>[6x]MAASTGYVRLWGAARCWVLRRPMLAAAGGRVPTAAGAWLLRGQRTCDASPPWALWGRGPAIGGQWRGFWEASSRGGGAFSGGEDASEGGAEEGAGGAGGSAGAGEGPVITALTPMTIPDVFPHLPLIAITRNPVFPRFIKIIEVKNKKLVELLRRKVRLAQPYVGVFLKRDDSNESDVVESLDEIYHTGTFAQIHEMQDLGDKLRMIVMGHRRVHISRQLEVEPEEPEAENKHKPRRKSKRGKKEAEDELSARHPAELAMEPTPELPAEVLMVEVENVVHEDFQVTEEVKALTAEIVKTIRDIIALNPLYRESVLQMMQAGQRVVDNPIYLSDMGAALTGAESHELQDVLEETNIPKRLYKALSLLKKEFELSKLQQRLGREVEEKIKQTHRKYLLQEQLKIIKKELGLE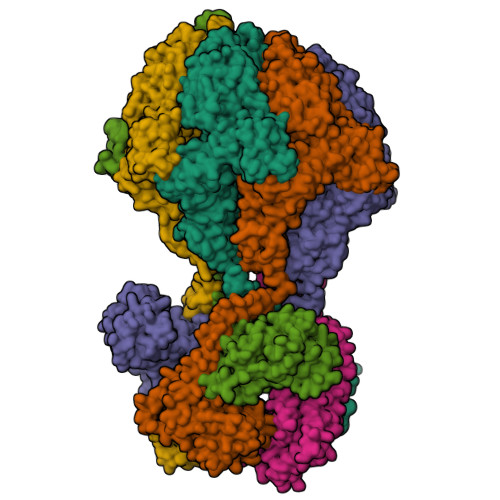KDDKDAIEEKFRERLKELVVPKHVMDVVDEELSKLGLLDNHSSEFNVTRNYLDWLTSIPWGKYSNENLDLARAQAVLEEDHYGMEDVKKRILEFIAVSQLRGSTQGKILCFYGPPGVGKTSIARSIARALNREYFRFSVGGMTDVAEIKGHRRTYVGAMPGKIIQCLKKTKTENPLILIDEVDKIGRGYQGDPSSALLELLDPEQNANFLDHYLDVPVDLSKVLFICTANVTDTIPEPLRDRMEMINVSGYVAQEKLAIAERYLVPQARALCGLDESKAKLSSDVLTLLIKQYCRESGVRNLQKQVEKVLRKSAYKIVSGEAESVEVTPENLQDFVGKPVFTVERMYDVTPPGVVMGLAWTAMGGSTLFVETSLRRPQDKDAKGDKDGSLEVTGQLGEVMKESARIAYTFARAFLMQHAPANDYLVTSHIHLHVPEGATPKDGPSAGCTIVTALLSLAMGRPVRQNLAMTGEVSLTGKILPVGGIKEKTIAAKRAGVTCIVLPAENKKDFYDLAAFITEGLEVHFVEHYREIFDIAFPDEQAEALAVER>[2x]MVIDGWTEEQHEPTVRHERPAAPQDVRRVMLLGSAEPSRELAIALQGLGAEVIAVDGYVGAPAHRIADQSVVVTMTDAEELTAVIRRLQPDFLVTVTAAVSVDALDAVEQADGECTELVPNARAVRCTADREGLRRLAADQLGLPTAPFWFVGSLGELQAVAVHAGFPLLVSPVAGVAGQGSS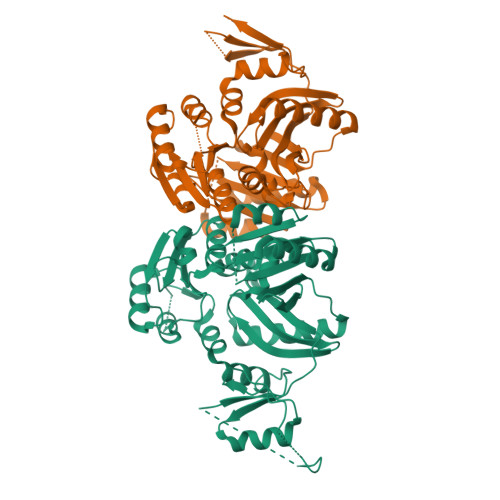VVAGPNEVEPAWQRAAGHQVQPQTGGVSPRVCAESVVEIEFLVTMIVVCSQGPNGPLIEFCAPIGHRDADAGELESWQPQKLSTAALDAAKSIAARIVKALGGRGVFGVELMINGDEVYFADVTVCPAGSAWVTVRSQRLSVFELQARAILGLAVDTLMISPGAARVINPDHTAGRAAVGAAPPADALTGALGVPESDVVIFGRGLGVALATAPEVAIARERAREVASRLNVPDSRE>KGPNLTEISKKITDSNAVLLAVKEVEALLSSIDELAKAIGKKIKNDGSLGDEANHNESLLAGAYTISTLITQKLSKLNGSEGLKEKIAAAKKCSEEFSTKLKDNHAQLGIQGVTDENAKKAILKANAAGKDKGVEELEKLSGSLESLSKAAKEMLANSVKELTSP[2x]

Outer surface protein C (OspC) plays a pivotal role in mediating tick-to-host transmission and infectivity of the Lyme disease spirochete, Borreliella burgdorferi. OspC is a helical-rich homodimer that interacts with tick salivary proteins, as well as components of the mammalian immune system. OspC consists of four long α-helices, two shorter α-helices (4 and 5), and two short antiparallel β-strands located between α1 and α2 (23, 24). The biologically functional molecule is a dimer (with monomers referred to here as OspC-OspC′) that assumes a knob-shaped structure anchored via an N-terminal lipidated moiety in the spirochete’s outer membrane.

To elucidate the structural basis for B5 IgG’s specificity for OspCA, we solved the crystal structures of recombinant OspCB and OspCK at 1.5-Å and 1.9-Å resolution, respectively, in the P21 space group. A deletion at residue 74 and an insertion of residue 165 in OspCB relative to OspCA and OspCK accounts for the greater structural deviation of OspCB to OspCA and OspCK, as exhibited by an RMSD of 0.9 Å for all atoms when the OspCB monomer was superposed onto OspCA or OspCK monomers. Superpositioning the B5-OspCA complex onto OspCB and OspCK revealed additional structural attributes that likely account for B5’s inability to recognize OspCB and OspCK. In OspCB and OspCK, Glu-175 is superposed with OspCA Gly-174. The bulkier and negatively charged Glu-175 side would be expected to clash (sterically and electrostatically) with Trp-100, thereby impeding B5 interaction. Furthermore, in the case of OspCB, an “insertion” of Ala-162 within loop 5-6 relative to OspCA alters the configuration of the loop, resulting in a theoretical clash of B5 with Tyr-47. OspCB is also unable to H-bond with B5 Tyr-47, due to an Ala rather than a Thr at position 162, as is the case in OspCA. Another structural feature in OspCB disfavoring B5 binding includes deletion of one residue immediately before Lys-74 in OspCB. This deletion substantially altered residue positions 73 to 75 within α-helix 1 of OspCB relative to the same residues in OspCA and OspCK. As a result, the superposed side chain of Lys-74 in OspCB clashes with B5 Tyr-102.> EEGLDFPEYDGVDRVINVNAKNYKNVFKKYEVLALLYHEPPEDDKASQRQFEMEELILELAAQVLEDKGVGFGLVDSEKDAAVAKKLGLTEEDSIYVFKEDEVIEYDGEFSADTLVEFLLDVLEDPVELIEGERELQAFENIEDEIKLIGYFKNKDSEHYKAFKEAAEEFHPYIPFFATFDSKVAKKLTLKLNEIDFYEAFMEEPVTIPDKPNSEEEIVNFVEEHRRSTLRKLKPESMYETWEDDMDGIHIVAFAEEADPDGYEFLEILKSVAQDNTDNPDLSIIWIDPDDFPLLVPYWEKTF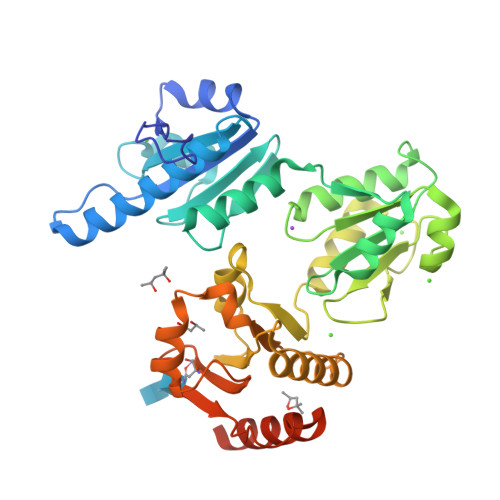DIDLSAPQIGVVNVTDADSVWMEMDDEEDLPSAEELEDWLEDVLEGEINTEDDDDEDDDDDDDD> 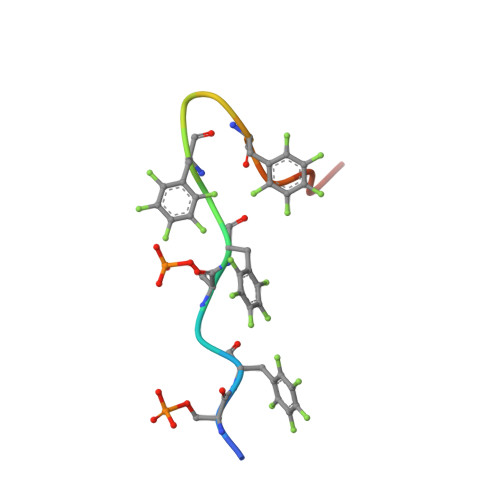PSFDSFDFEDFPAALWX>[60x]MGSSHHHHHHSSSAALEVLFQGPMELFNRVGRVLKSQLTHWQQQQEAPEDLLERLLGEMELELIELRRALAQTIATFKSTERQRDAQQLIAQRWYEKAQAALDRGNEQLAREALGQRQSYQSHTEALGKSLGEQRALVEQVRGQLQKLERKYLELKSQKNLYLARLKSAIAAQKIEEIAGNLDNASASSLFERIETKILELEAERELLNPPPSPLDKKFEQWEEQQAVEATLAAMKARRSLPPPSS

The bacterial member PspA is part of the phage shock protein (psp) response that maintains structural integrity of membranes under stress conditions such as temperature and infection. The main effector of the Psp system is PspA, a 25 kDa protein consisting of six α-helices connected by short loops and an elongated hairpin, where the N-terminal helix α0 of the protein remains unfolded in the absence of membranes. Interestingly, PspA is related to eukaryotic and archaeal endosomal sorting complexes required for transport (ESCRT)-III proteins and has a similar structure. Here, we show that rods of bacterial ESCRT-III protein PspA internalize and thin membrane tubules by overcoming the required bending energy through progressive membrane binding of the N-terminal helix in the PspA assembly.

For our analyses, we refolded PspA in the presence of 50 nm sized small unilamellar EPL vesicles, similar to a recently described protocol. In the presence of EPL membranes, the rods had a wider diameter and a broader diameter distribution (200 to 345 Å) in comparison with the diameter values and distribution of the previously analyzed apo protein (180 to 290 Å). By segmenting the rods of the EPL-PspA sample and sorting the segments according to diameter through classification, we determined a total of 10 cryo-EM structures with resolutions ranging from 4.7 to 6.5 Å. While the imposed helical symmetry parameters suggested no architectural relationship between the PspA rods, helical lattice plots revealed that the left-handed helical rung corresponding to layer line ~110 Å in the power spectrum increased in Bessel order from n = 10, 11, 12…18 with increasing diameters of 200, 215, 235…345 Å, respectively. Upon insertion of an additional subunit into the helical rung, the assembly widens in discrete steps of around 20 Å up to a diameter of 345 Å. The rods with diameters larger than 280 Å were of particular interest as they showed enclosed double-layered lipid density in the cross-sectional top and side views in addition to the expected PspA protein densities, whereas rods of 270 Å diameter contained only partial lipid density and smaller diameters showed no density in the cross-section views. When comparing them with the previous apo structures, we observed that the structures of the EPL sample were identical to the apo structures with the same diameters, including their respective helical symmetry. The cryo-EM structures and MD simulations showed that only rods wider than 270 Å internalize and tubulate membranes. As indicated in the simulations, the energy required for membrane bending likely is too high for thinner rods to bend and internalize membrane tubules.>SVKLAGNSSLCPVSGWAIYSKDNSVRIGSKGDVFVIREPFISCSPLECRTFFLTQGALLNDKHSNGTIKDRSPYRTLMSCPIGEVPSPYNSRFESVAWSASACHDGINWLTIGISGPDNGAVAVLKYNGIITDTIKSWRNNILRTQESECACVNGSCFTVMTDGPNNGQASYKIFRIEKGKIVKSVEMNAPNYHYEECSCYPDSSEITCVCRDNWHGSNRPWVSFNQNLEYQIGYICSGIFGDNPRPNDKTGSCGPVSSNGANGVKGFSFKYGNGVWIGRTKSISSRNGFEMIWDPNGWTG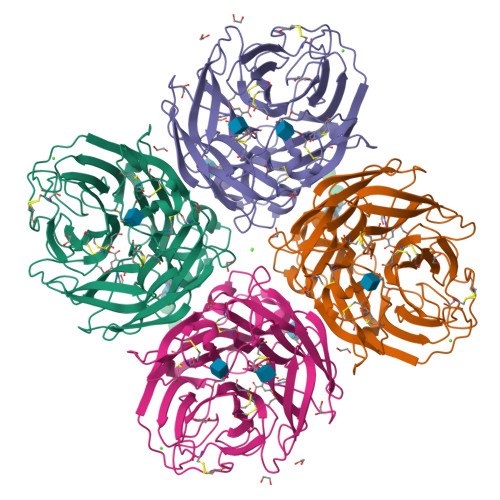TDNNFSIKQDIVGINEWSGYSGSFVQHPELTGLDCIRPCFWVELIRGRPKENTIWTSGSSISFCGVNSDTVGWSWPDGAELPFTIDK[2x]>[2x]MSNDDNVELTDGFHVLIDALKMNDIDTMYGVVGIPITNLARMWQDDGQRFYSFRHEQHAGYAASIAGYIEGKPGVCLTVSAPGFLNGVTSLAHATTNCFPMILLSGSSEREIVDLQQGDYEEMDQMNVARPHCKASFRINSIKDIPIGIARAVRTAVSGRPGGVYVDLPAKLFGQ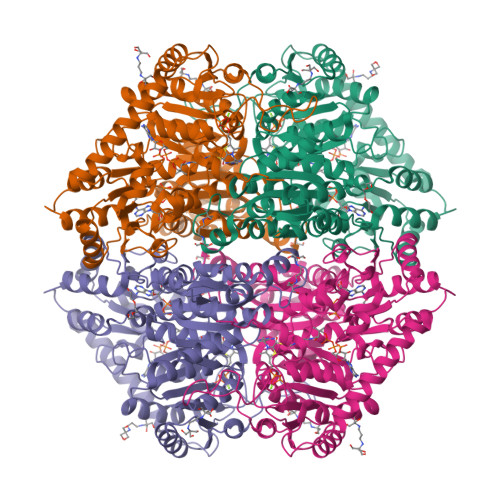TISVEEANKLLFKPIDPAPAQIPAEDAIARAADLIKNAKRPVIMLGKGAAYAQCDDEIRALVEETGIPFLPMGMAKGLLPDNHPQSAAATRAFALAQCDVCVLIGARLNWLMQHGKGKTWGDELKKYVQIDIQANEMDSNQPIAAPVVGDIKSAVSLLRKALKGAPKADAEWTGALKAKVDGNKAKLAGKMTAETPSGMMNYSNSLGVVRDFMLANPDISLVNEGANALDNTRMIVDMLKPRKRLDSGTWGVMGIGMGYCVAAAAVTGKPVIAVEGDSAFGFSGMELETICRYNLPVTVIIMNNGGIYKGNEADPQPGVISCTRLTRGRYDMMMEAFGGKGYVANTPAELKAALEEAVASGKPCLINAMIDPDAGVESGRIKSLNVVSKVGKK>GMATE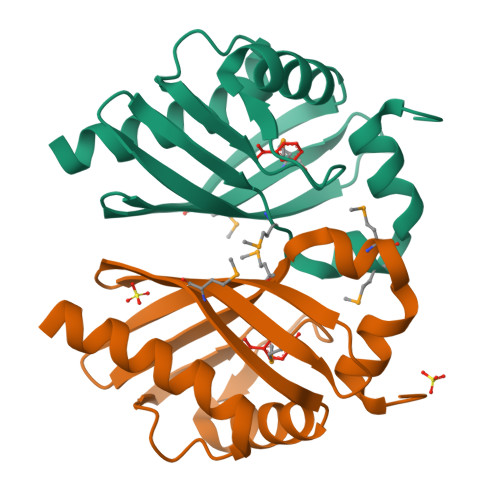KYHEILKKYFLSFETGDFSQVQFSCNLEFLSPISGNTLKGTEEVIPFLKGVTTRVAEVNIMSTTVEYPRASGVWQMRTTKGTLYTLHNFFRLDEEGIVYVWPMFDPKAVMENPDALIQWLTGKDY[4x]>MGHHHHHHGGSENLYFQGNEDILKASATQSAVAGTYQIQVNSLATSSKIALQAIADPANAKFNSGTLNISVGDTKLPAITVDSSNNTLAGMRDAINQAGKEAGVSATIITDNSGSRLVLSSTKTGDGKDIKVEVSDDGSGGNTSLSQLAFDPATAPKLSDGAAAGYVTKAANGEITVDGLKRSIASNSVSDVIDGVSFDVKAVTEAGKPITLTVSRDDAGVKDNVKKFVEAYNTLTKFINEQTVVTKVGEDKNPVTGALLGDASVRALVNTMRSELIASNENGSVRNLAALGITTTKDGTLEIDEKKLDKAISADFEGVASYFTGDTGLAKRLGDKMKPYTDAQGI[2x]

Flagella are helix-shaped hollow attachments formed predominantly by thousands of copies of the protein flagellin (also called FliC), anchored in the bacterial membrane by a hook (or joint) that is attached to the basal body and that is composed of rotary motor proteins. A FliD (also called HAP2) oligomer forms the cap protein complex that is located at the tip of the flagellar filament. This complex controls the distal growth of the filament by regulating the assembly of FliC molecules, which are transported through the hollow filament from the cytoplasm to the tip of the flagellum. Flagellum-mediated motility is crucial for the virulence and pathogenicity of numerous bacteria, including Campylobacter jejuni, Salmonella, Escherichia coli, Vibrio cholera, and Pseudomonas aeruginosa, as well as the major causative agent of gastric cancer Helicobacter pylori.

We improved initially weakly diffracting crystals of FliD78–405 by random matrix microseed screening, yielding crystals that diffracted to 2.2 Å resolution. Our crystal structure of FliD78–405 reveals that it consists of two discreet regions with distinct conformational properties, corresponding to a stable head region and a flexible and/or disordered leg region. Residues 80–101 form two β strands that belong to the first domain (Head 1), the second domain (Head 2) is formed in its entirety by the contiguous residues 104–230, and residues 231–273 then complete the first domain. Despite this, we were able to model the initial α helical structural element, corresponding to residues 274–308, of this region. This helix extends from the axis of the head region at a nearly perpendicular angle, resulting in an L-shaped monomer subunit structure. In the crystal, FliD78–405 monomer subunits are arranged in hexamers, resulting in a shape akin to a six-pointed star when viewed from the top of the FliD oligomer, which corresponds to the distal end of the growing flagellum. When viewed from the side, the FliD hexamer appears as a six-legged stool, the legs of which extend 55 Å below the bottom of the head region. The leg-to-leg stacking forms dodecamers, resulting from the helix–helix interaction of the residues 274–302 of stacked molecules and the interaction of residues 303–308 of one FliD78–405 molecule with Head 1 domain of a stacked molecule, burying a surface area of 1362 Å2. Although the FliD78–405 crystal structure exhibits intermolecular contacts between the head regions of FliD78–405 subunits comprising the hexamer, each of these interfaces is small, with a buried surface area of only 665 Å2, and contains few intermolecular contacts relative to typical protein–protein interactions. Second, despite vanishingly low sequence similarity, each domain within the head region exhibits high structural similarity to the corresponding domains of other flagellar proteins, including the hook-filament junction protein/FlgK and flagellin/FliC.> GCTGGAAATTTCC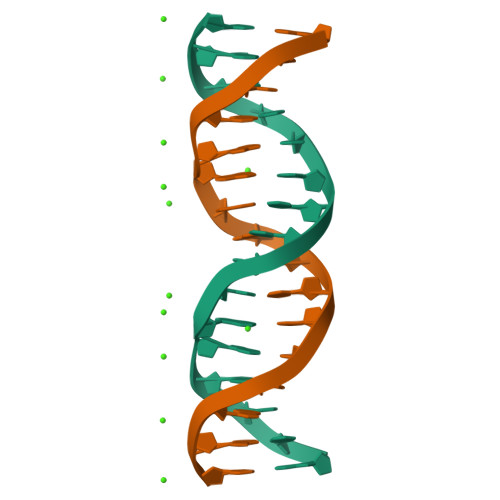AGC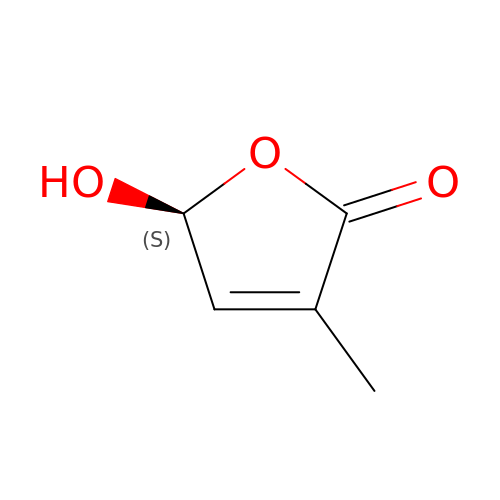(5S)-5-hydroxy-3-methylfuran-2(5H)-one | C5 H6 O3 | HQIZYPQNJWENRT-BYPYZUCNSA-N>MSSGATPSNVVLVGKKPVMNYVLAALTLLNQGVSEITIKARGRAISKAVDTVEIVRNRALPDKIEVKEIRIGSQVVTSQDGRQSRVSTIEIGIRKKA[2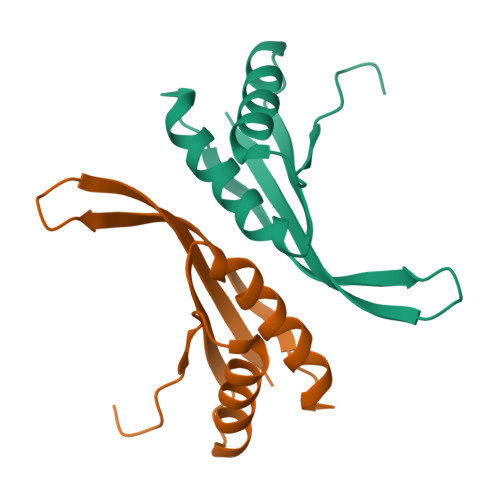x]>[2x]GSANLKNKTLVVTTILSNPYCMRKESAIPLSGNDQFEGYAVDLIHEISKSLGFNYKIQLVPDGSYGSLNKLTGEWNGMIRELLEQRADLAIADLTITFEREQAVDFTTPFMNLGVSILYRKGTPIESAEDLAKQTRIKYGALKGGSTAAFFRDSKISTYQRMWSFMESAR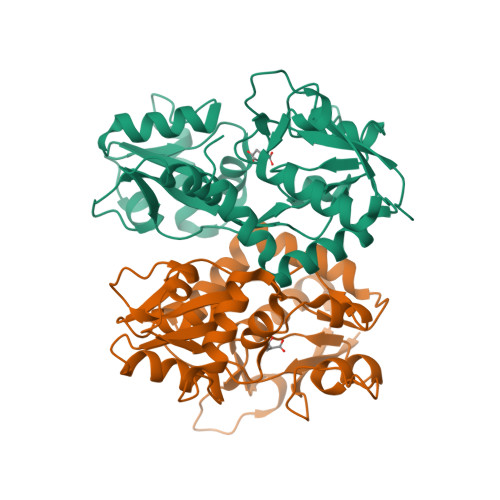PSVFTASNGEGVERVAKGKGSYAFLMESTSIEYVTERNCELTQVGGMLDTKSYGIATPPNSPYRTAINSVILKLQEEGKLHILKTKWWKEKRGGGKCR>SANDKQYISYNNVHQLCQVSAERIKNFKPDLIIAIGGGGFIPARILRTFLKEPGVPTIRIFAIILSLYEDLNSVGSEVEEVGVKVSRTQWIDYEQCKLDLVGKNVLIVDEVDDTRTTLHYALSELEKDAAEQAKAKGIDTEKSPEMKTNFGIFVLHDKQKPKKADLPAEMLNDKNRYF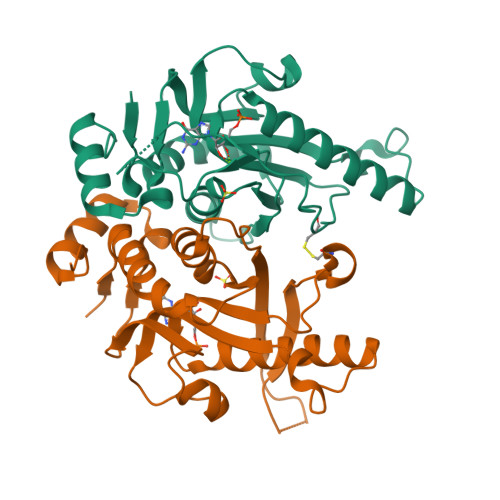AAKTVPDKWYAYPWESTDIVFHTRMAIEQGNDIFI[2x]>MGSDKIHHHHHHENLYFQQDTEKKVSEEGFVFTTVKENPITS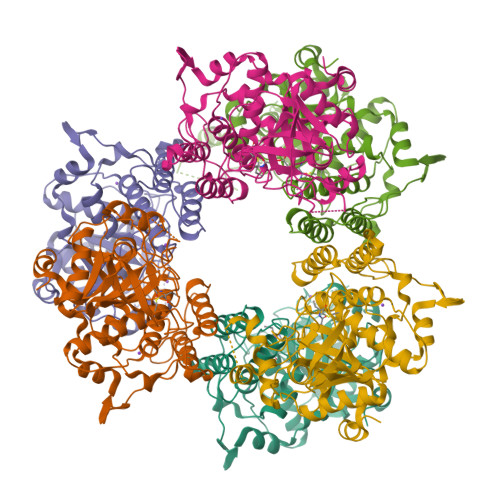VKNQNRAGTCWCYSSYSFLESELLRMGKGEYDLSEMFTVYNTYLDRADAAVRTHGDVSFSQGGSFYDALYGMETFGLVPEEEMRPGMMYADTLSNHTELSALTDAMVAAIAKGKLRKLQSDENNAMLWKKAVAAVHQIYLGVPPEKFTYKGKEYTPKSFFESTGLKASDYVSLTSYTHHPFYTQFPLEIQDNWRHGMSYNLPLDEFMEVFDNAINTGYTIAWGSDVSESGFTRDGVAVMPDDEKVQELSGSDMAHWLKLKPEEKKLNTKPQPQKWCTQAERQLAYDNYETTDDHGMQIYGIAKDQEGNEYYMVKNSWGTNSKYNGIWYASKAFVRYKTMNIVVHKDALPKAIKAKLGIK[6x]> MVPISPIETVPVKLKPGMDGPKVKQWPLTEE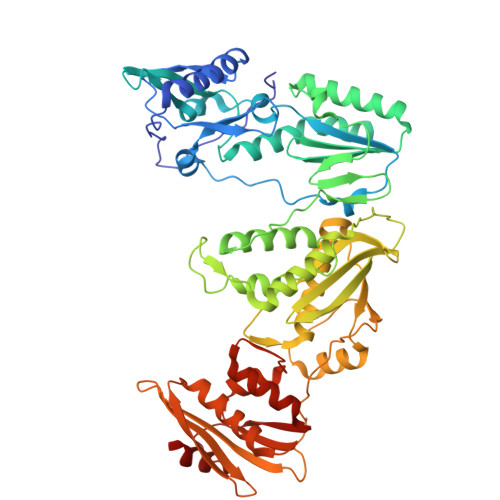KIKALVEICTEMEKEGKISKIGPENPYNTPVFAIKKKDSTKWRKLVDFRELNKRTQDFWEVQLGIPHPAGLKQKKSVTVLDVGDAFYSVPLDKDFRKYTAFTIPSINNETPGIRYQYNVLPMGWKGSPAIMQSSMTKILEPFRKQNPDIVIYQYVDDLYVGSDLEIGQHRTKIEELRQHLLRWGFTTPDKKHQKEPPFLWMGYELHPDKWTVQPIVLPEKDSWTVNDIQKLVGKLNWASQIYAGIKVRQLSKLLRGTKALTEVVPLTEEAELELAENREILKEPVHGVYYDPSKDLIAEIQKQGQGQWTYQIYQEPFKNLKTGKYARMKGAHTNDVKQLTEAVQKIATESIVIWGKTPKFKLPIQKETWEAWWTEYWQATWIPEWEFVNTPPLVKLWYQLEKEPIIGAETFYVDGAANRETKLGKAGYVTDRGRQKVVPLTDTTNQKTELQAIHLALQDSGLEVNIVTDSQYALGIIQAQPDKSESELVSQIIEQLIKKEKVYLAWVPAHKGIGGNEQVDKLVSAG3-AMINO-N-METHYL-6-[3-(1H-TETRAZOL-5-YL)PHENYL]PYRAZINE-2-CARBOXAMIDE | C13 H12 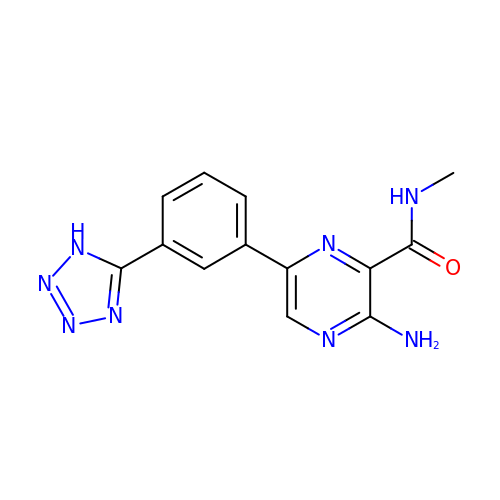N8 O | PLUDSXLHMVRUKP-UHFFFAOYSA-N>CGSIVPRREWRALASECRERLTRPVRYVVVSHTAGSHCDTPA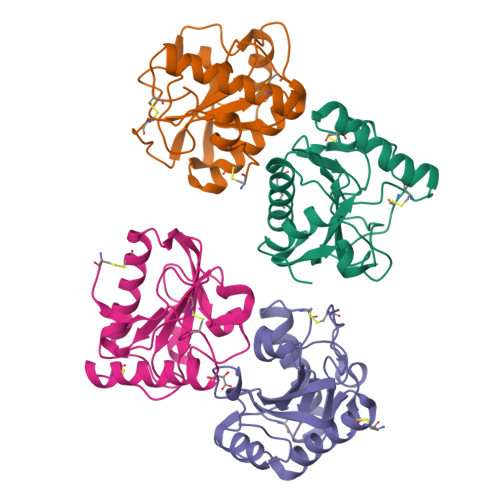SCAQQAQNVQSYHVRNLGWCDVGYNFLIGEDGLVYEGRGWNIKGAHAGPTWNPISIGISFMGNYMNRVPPPRALRAAQNLLACGVALGALRSNYEVKGHRDVQPTLSPGDRLYEIIQTWSHYRA[4x]> MGLEERLPGGILLSTVETVAGYVRKGSLWPATFGLACCAIEMMSTAGPRF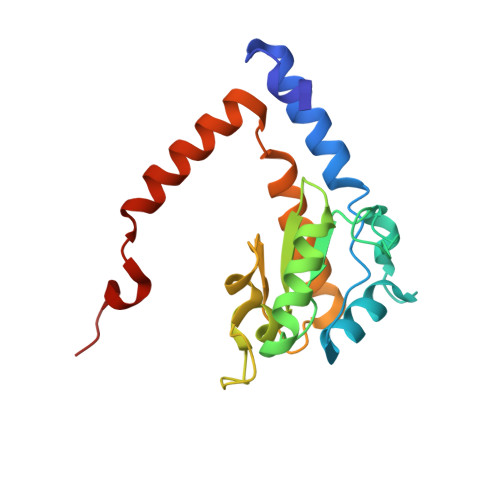DIARFGMERFSATPRQADLMIVAGRVSQKMAPVLRQIYDQMVEPKWVLAMGVCASSGGMFNNYAVVQGVDHVVPVDIYLPGCPPRPEMLLHAILKLHDKIQQMPLGVNREEAIREAEQAALAVPPTIELKGLLR5'-CHLORO-5'-DEOXYADENOSINE 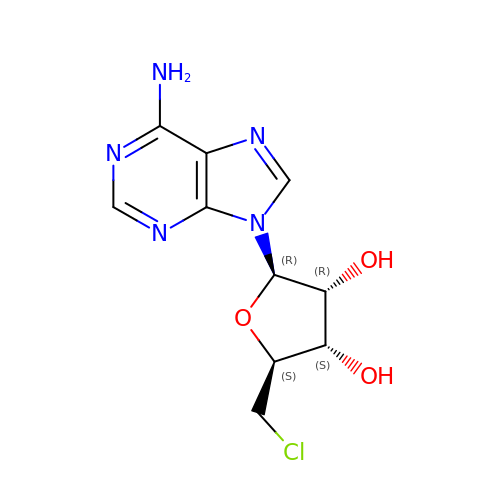| C10 H12 Cl N5 O3 | IYSNPOMTKFZDHZ-KQYNXXCUSA-N>[3x]AYLLFYTE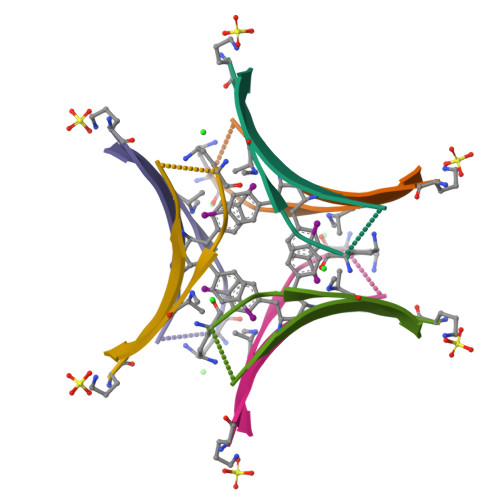AKVAAAVK> ADTIVAVELDTYPNTDIGDPNYPHIGIDIKSIRSKKTTRWNIQNGKVGTAHINYNSVGKRLSAIVSYPNSDSATVSYDVDLDNVLPEWVRVGLSATTGLYKETNTILSWSFTSKLKSNSTADANALHFTFNQFSKDQKDLILQGDATTGTDGNLELTRVSSNGSPQGNSVGRALFYAPVHIWESSAVV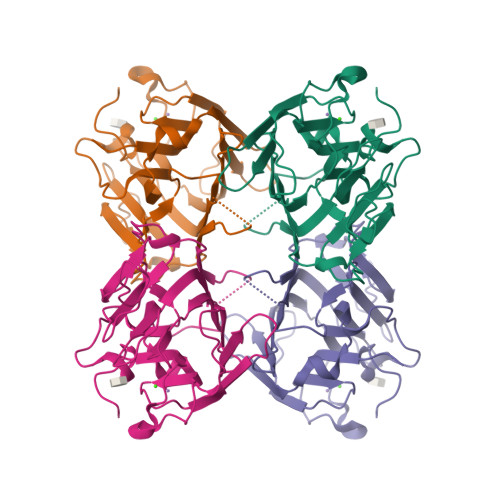ASFDATFKFLIKSPDSEPADGITFFIANIDSSIPSGSGGRLLGLFPDAN> GPGSGQEGSVCLRSSDCASGLCCARHFWSKICKPVL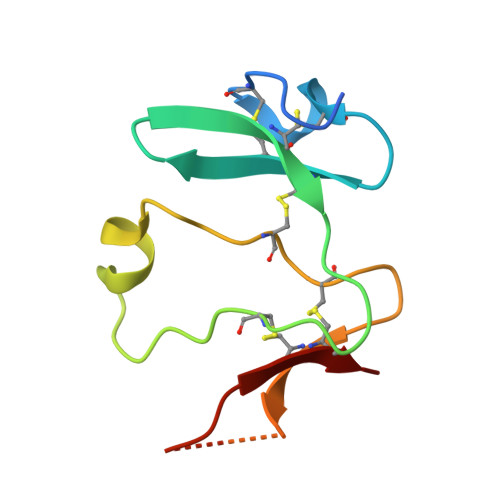KEGQVCTKHRRKGSHGLEIFQRCYCGEGLSCRIQKDHHQASNSSRLHTCQRH> MAYFDYTSAKPVDERILEAMLPYMTESFGNPSSVHSYGFKAREAVQEAREKVAKLVNGGGGTVVFTSGATEANNLAIIGYAMRNARKGKH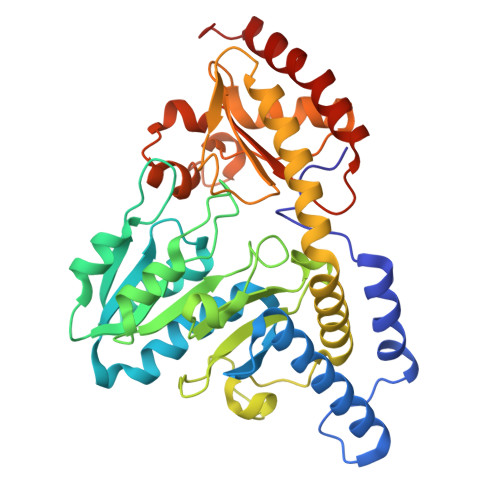ILVSAVEHMSVINPAKFLQKQGFEVEYIPVGKYGEVDVSFIDQKLRDDTILVSVQHANNEIGTIQPVEEISEVLAGKAALHIDATASVGQIEVDVEKIGADMLTISSNDIYGPKGVGALWIRKEAKLQPVILGGGQENGLRSGSENVPSIVGFGKAAEITAMEWREEAERLRRLRDRIIDNVLKIEESYLNGHPEKRLPNNVNVRFSYIEGESIVLSLDMAGIQASTGSACSSKTLQPSHVLMACGLKHEEAHGTLLLTLGRYNTDEDVDRLLEVLPGVIERLRSMSPLYRR>DRPSYCNLPADSGSGTKSEQRIYYNSARKQCLTFTYNGQGGNENNFRRTYDCRRT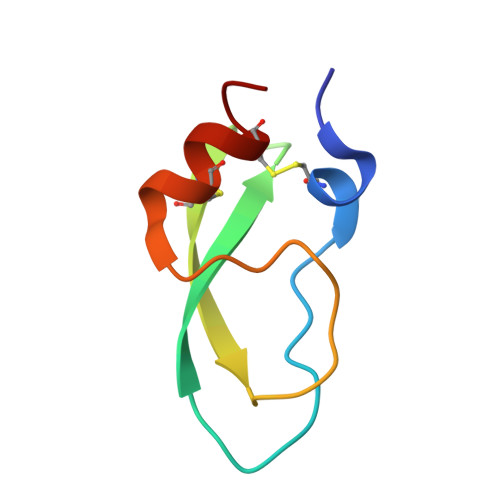CQYP[2x]> MAAQGFLLIATFLLVLMVLARPLGSGLARLINDIPLPGTTGVERVLFRALGVSDREMNWKQYLCAILGLNMLGLAVLFFMLLGQHYLPLNPQQLPGLSWDLALNTAVSFVTNTNWQSYSGETTLSYFSQMAGLTVQNFLSAASGIAVIFALIRAFTRQSMSTLGNAWVDLLRITLWVLVPVALLIALFFIQQGALQNFLPYQAVNTVEGAQQLLPMGPVASQEAIKMLGTNGGGFFNANSSHPFENPTALTNFVQMLAIFLIPTALCFAFGEVMGDRRQGRMLLWAMSVIFVICVGVVMWAEVQGNPHLLALGTDSSINMEGKESRFGVLVSSLFAVVTTAASCGAVIAMHDSFTALGGMVPMWLMQIGEVVFGGVGSGLYGMMLFVLLAVFIAGLMIGRTPEYLGKKIDVREMKLTALAIL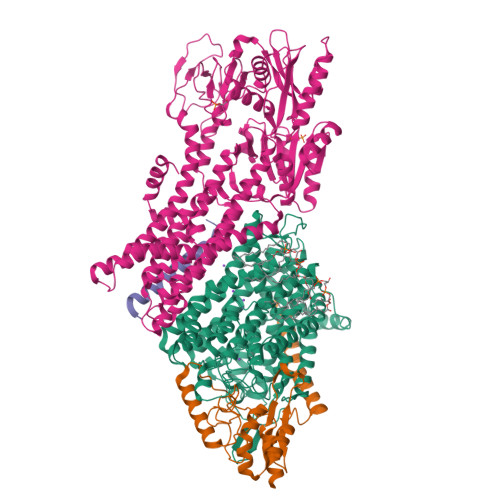VTPTLVLMGAALAMMTDAGRSAMLNPGPHGFSEVLYAVSSAANNNGSAFAGLSANSPFWNCLLAFCMFVGRFGVIIPVMAIAGSLVSKKSQAASSGTLPTHGPLFVGLLIGTVLLVGALTFIPALALGPVAEYLS;> MSRKQLALFEPTLVVQALKEAVKKLNPQAQWRNPVMFIVWIGSLLTTCISIAMASGAMPGNALFSAAISGWLWITVLFANFAEALAEGRSKAQANSLKGVKKTAFARKLREPKYGAAADKVPADQLRKGDIVLVEAGDIIPCDGEVIEGGASVDESAITGESAPVIRESGGDFASVTGGTRILSDWLVIECSVNPGETFLDRMIAMVEGAQRRKTPNEIALTILLIALTIVFLLATATLWPFSAWGGNAVSVTVLVALLVCLIPTTIGGLLSAIGVAGMSRMLGANVIATSGRAVEAAGDVDVLLLDKTGTITLGNRQASEFIPAQGVDEKTLADAAQLASLADETPEGRSIVILAKQRFNLRERDVQSLHATFVPFTAQSRMSGINIDNRMIRKGSVDAIRRHVEANGGHFPTDVDQKVDQVARQGATPLVVVEGSRVLGVIALKDIVKGGIKERFAQLRKMGIKTVMITGDNRLTAAAIAAEAGVDDFLAEATPEAKLALIRQYQAEGRLVAMTGDGTNDAPALAQADVAVAMNSGTQAAKEAGNMVDLDSNPTKLIEVVHIGKQMLMTRGSLTTFSIANDVAKYFAIIPAAFAATYPQLNALNIMCLHSPDSAILSAVIFNALIIVFLIPLALKGVSYKPLTASAMLRRNLWIYGLGGLLVPFIGIKVIDLLLTVCGLV;> MSGLRPALSTFIFLLLITGGVYPLLTTVLGQWWFPWQANGSLIREGDTVRGSALIGQNFTGNGYFHGRPSATAEMPYNPQASGGSNLAVSNPELDKLIAARVAALRAANPDASASVPVELVTASASGLDNNITPQAAAWQIPRVAKARNLSVEQLTQLIAKYSQQPLVKYIGQPVVNIVELNLALDKLDE;> MSAGVITGVLLVFLLLGYLVYALINAE> ADYDLKFGMNAGTSSNEYKAAEM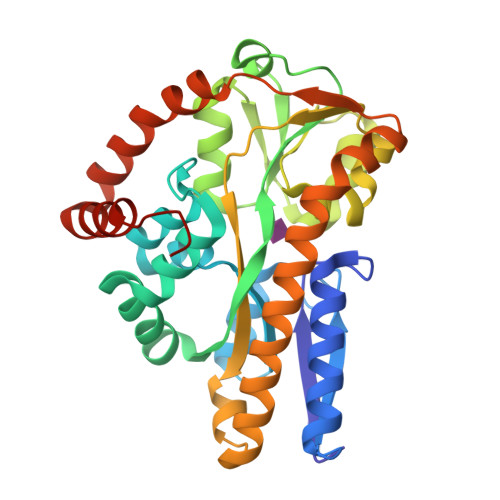FAKEVKEKSQGKIEISLYPSSQLGDDRAMLKQLKDGSLDFTFAESARFQLFYPEAAVFALPYVISNYNVAQKALFDTEFGKDLIKKMDKDLGVTLLSQAYNGTRQTTSNRAINSIADMKGLKLAVPNAATNLAYAKYVGASPTPMAFSEVYLALQTNAVDGQENPLAAVQAQKFYEVQKFLAMTNHILNDQLYLVSNETYKELPEDLQKVVKDAAENAAKYHTKLFVDGEKDLVTFFEKQGVKITHPDLVPFKESMKPYYAEFVKQTGQKGESALKQIEAINPHHHHHH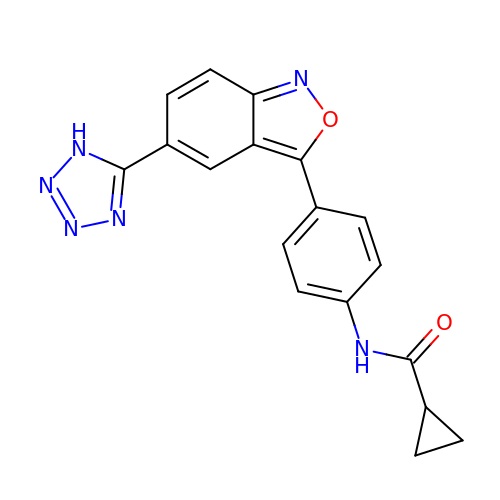N-{4-[(5P)-5-(1H-tetrazol-5-yl)-2,1-benzoxazol-3-yl]phenyl}cyclopropanecarboxamide | C18 H14 N6 O2 | AXQAWOHSTLOJBL-UHFFFAOYSA-N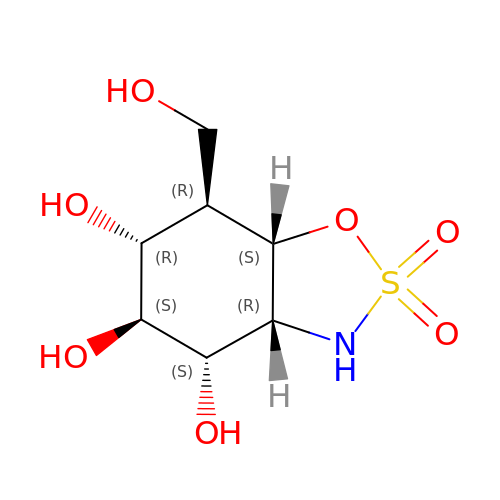(3aR,4S,5S,6R,7R,7aS)-7-(hydroxymethyl)-2,2-bis(oxidanylidene)-3a,4,5,6,7,7a-hexahydro-3H-benzo[d][1,2,3]oxathiazole-4,5,6-triol | C7 H13 N O7 S | LDXSPHJOJCEWFB-MAFUWASYSA-N>MGSSHHHHHHSSGMSLPTAEAVRTIRYGLIGAGHMAREHVRNLALIPGSLITAVSDPQPSSLEETVAEIGYEVTTFPDHRELLVSGLVDALVIASPNDTHLDILKDIFSNQMKLPVLVEKPVCTTAAQADELESLAAGYSAPVWVAMEYRYMPPVQELIQAAHGGKLGNVFMLSIVEHRFPFLHKVDAWNRFNERTGGTLVEKCCHFFDLMRLILQDEPTRIYASGGHDVNHMDELYEGRVSDMIDNAYVVVDFKSGRRAMLELSMFAEGSKFQERISIVGDAAKIECLIPVAASHWIEGDESEAVVEFSPRSPLGPETHEVPVDEAVLAAGAHHGSTYYEHLGYRKAILGEGPVEVTVADGLQSVRMGLAAERSIIEGRPVELLSANSAVS[2x]

Here, we identify an alternative approach to sulfoquinovoside hydrolysis that is adopted by these organisms and discover a family of SQases belonging to a new glycoside hydrolase family (GH188). These new SQases operate through an oxidoreductive mechanism that results in net hydrolysis and involves a catalytic NAD+ cofactor. The SqgA proteins adopt a two-domain fold with an N-terminal dinucleotide binding Rossmann domain and a C-terminal α/β dimerization domain. The structures reveal homodimers, consistent with molar mass analysis using size-exclusion chromatography-multiangle laser light scattering in solution.

Soaking and cocrystallization experiments provided structures of the ArSqgA·NAD+·SQ and FlSqgA·NAD+·SQ complexes, which diffracted to 2.4 and 2.3 Å, respectively. Both ternary complexes were essentially identical, with respect to the active site interactions. In the ArSqgA·NAD+·SQ complex, SQ is situated above the nicotinamide ring, with C3 of SQ 3.4 Å away from C4 of the nicotinamide ring, at an appropriate distance for hydride transfer and oxidation of C3 of an SQ glycoside. A range of specific interactions occur with the hydroxyl groups of SQ: C1–OH at 2.5 Å from His321 and a water molecule; C2-OH with Tyr136 (2.6 Å); C3–OH with His193 (2.7 Å) and Lys107 (2.6 Å); and C4–OH with Glu189 (2.6 Å). The characteristic 6-sulfonate group of SQ engages in a triad of interactions in the ArSqgA·NAD+·SQ: one oxygen H-bonds to Arg166 (2.6 Å), a second to Lys172 (2.9 Å), and a third to the backbone amide of Leu170 (2.8 Å). Superposition of ArSqgA·NAD+ binary and ArSqgA·NAD+·SQ ternary complexes (backbone RMSD of 0.5 Å over 364 residues) revealed no major structural changes upon binding SQ. The active site was also largely unchanged with the notable exception of the Tyr136 residue in some of the individual protomer chains, which rotated 72° about the Cα–Cβ bond to engage with C2–OH of SQ in the ArSqgA·NAD+·SQ complex. All of these residues are conserved across the studied SqgA homologues. Superposition of the ArSqgA·NAD+·SQ and AmGH109A·NAD+·GalNAc complexes shows that His259 (His193 in ArSqgA) and His404 (His321 in ArSqgA) are structurally conserved. However, a difference occurs in the active site with respect to the location of Tyr226 of AmGH109A, where Glu163 occupies the equivalent position in ArSqgA; and Tyr136 hydrogen-bonds to C2–OH of SQ in our structure, implicating it in catalysis.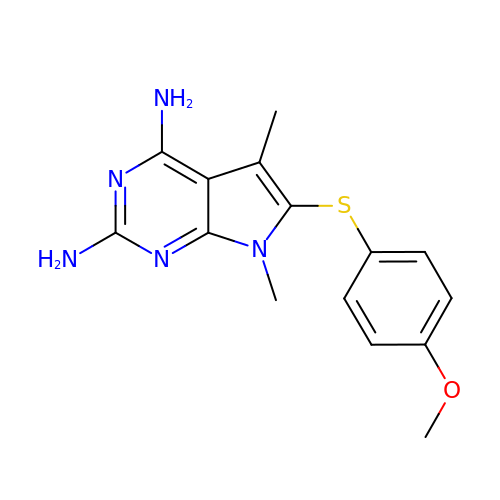6-[(4-methoxyphenyl)sulfanyl]-5,7-dimethyl-7H-pyrrolo[2,3-d]pyrimidine-2,4-diamine | C15 H17 N5 O S | OKWZEJPRXOZLRD-UHFFFAOYSA-N Phytases (myo-inositol hexakisphosphate phosphohydrolases) catalyse the hydrolysis of phytate into inorganic phosphate (Pi) and lower phosphorylated myo-inositols. Here we report the identification of two HAPPs from the enterobacteria Hafnia alvei (HaPhy) and Yersinia kristensenii (YkPhy), together with biochemical studies of their pH and temperature optima, as well as their phytate degradation pattern, which show that they are 6-phytases. The enzymes share a common catalytic site architecture located at the interface of the two domains involving the conserved N-terminal active site motif RHGXRXP and the C-terminal HD. The two-step reaction involves a nucleophilic attack on the phosphorous by the histidine from the RHGXRXP motif to form a covalent phosphohistidine intermediate while the aspartic acid of the HD motif serves as a proton donor to the oxygen atom of the scissile phosphomonoester bond.

The structure of Pi-YkPhy was refined at a resolution of 1.67 Å with two protein monomers in the asymmetric unit, each modelled with residues 6 to 414, and with very similar folds (rmsd = 0.22 Å). The overall fold is essentially identical to that of apo-HaPhy (rmsd = 0.96 Å over 391 residues) and is shown in Fig. S6 in the same orientation as for HaPhy in Fig. 5(a). Each monomer contains two Pi molecules in its active site. The first Pi superposes almost perfectly with the 6-sulphate from the HaPhy-MIHS complex. The second is coordinated by His126 (corresponding to His128 in HaPhy) similar to the 1-sulphate of MIHS, but does not superimpose with any of sulphates of the MIHS ring. The YkPhy structure is very similar to that of HaPhy, with a very close overlap of the active site residues, suggesting that it is also a 6-phytase in accordance with our biochemical data.

>[2x]MTVAKKYLRLSVLTLVLSSFTLSAAPLAAQSTGYTLERVVILSRHGVRSPTKQTQLMNDVTPDKWPQWPVKAGYLTPRGAGLVTLMGGFYGDYFRSYGLLPAGCPADESIYVQADVDQRTRLTGQAFLDGIAPDCGLKVHYQADLKKIDPLFHTVEAGVCKLDPEKTHQAVEKRLGGPLNELSQRYAKPFALMGEVLNFSASPYCNSLQQKGKACDFATFAANEIEVNKEGTKVSLSGPLALSSTLGEIFLLQNSQAMPDVAWNRLSGEENWISLLSLHNAQFDLMAKTPYIARHKGTPLLQQIDTALVLQRDAQGQTLPLSPQTKLLFLGGHDTNIANIAGMLGANWQLPQQPDNTPPGGGLVFELWQNPDNHQRYVAVKMFYQTMEQLRNADKLDLKNNPARIVPIAIEGCENEGDNKLCQLETFQKKVAQVIEPSCHI> GPGSMSEKLQKVLARAGHGSRREIESIIEAGRVSVDGKIAKLGDRVEVTPGLKIRIDGHLISVRESAEQICRVLAYYKPEGELCTRNDPEGRPTVFDRLPKLRGARWIAVGRLDVNTCGLLLFTTDGELANRLMHPSREVEREYAVRVFGQVDDAKLRDLSRGVQLEDGPAAFKTIKFSGGEGINQWYNVTLTEGRNREVRRLWEAVGVQVSRLIRVRYGDIPLPKGLPRGGWTELDLAQTNYLRELVELPPETS

Isomerization of uridine to its C-glycoside isomer, pseudouridine (Ψ), is the most prevalent RNA modification. Here we address the question of how two homologous E. coli Ψ synthases, RluB and RluF, selectively modify adjacent bases on a stem-loop of E. coli 23S rRNA. RluB is specific for U2605 whereas RluF is selective for U2604, but also modifies U2605 to a small extent. RluB (1–251) is comprised of an N-terminal S4 domain (residues 1–60) connected by a flexible linker to a catalytic domain (residues 66–251).

The crystal structure of apo-RluB (1–251) was therefore solved to a resolution of 2.5 Å with one RluB molecule per asymmetric unit. The S4 domain (residues 1–60) is not visible in the structure of apo-RluB indicating that this domain is either disordered or flexible in the absence of RNA; flexibility between the S4 domain and the catalytic core has also been reported for the Ψ synthases RsuA and RluD. Apo-RluB is similar to apo-RluF with an rmsd of 1.9 Å (over 164 Cα) with a highly conserved core that encompasses the central beta sheet and helices α1–α3 (rmsd of 1.1 Å over 126 residues). Differences are localized to insertions of 1–4 residues in non-conserved loops on the periphery of the proteins, however there are two significant differences between the structures relevant to the different substrate specificities of RluF and RluB. First, the residues that form two C-terminal turns of helix α2 in RluF form a loop in RluB. Second, in RluB, helix α4 is followed by a hairpin turn that changes the direction of the peptide chain and allows it to pack against α4 instead of impinging on the bulge-binding site. In the apo-RluB structure residues 131–138 form a loop, whereas in the apo-RluF structure these residues are a two-turn extension of a helix (α2 in RluF) that directly overlaps the bulge-binding site. There are three major conformational changes to RluB that occur upon RNA binding. Superposition of the apo-RluB and the RNA-bound RluB structures results in a large rmsd of 2.1 Å (over 185 Cαs), however individually the subdomains align closely. Finally, residues 132–134 in the loop between α1 and β4 refold into a 310 helix and bind to the RNA near the bulge.> MANMKNSNDRIILFRKAGEKVDATKMLFLTEYGLSHEADTDTEDTMDGSYNTGGSVESTMSGTAKMFYGDD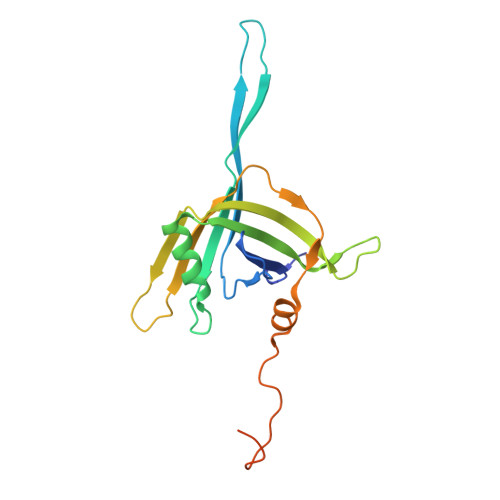FADEIEDAVVDRVLYEAWEVESRIPGKNGDSAKFKAKYFQGFHNKFELKAEANGIDEYEYEYGVNGRFQRGFATLPEAVTKKLKATGYRFHDTTKEDALTSEDLTAIPQPKVDSSTVTPGEV> TRSGKVMRRLL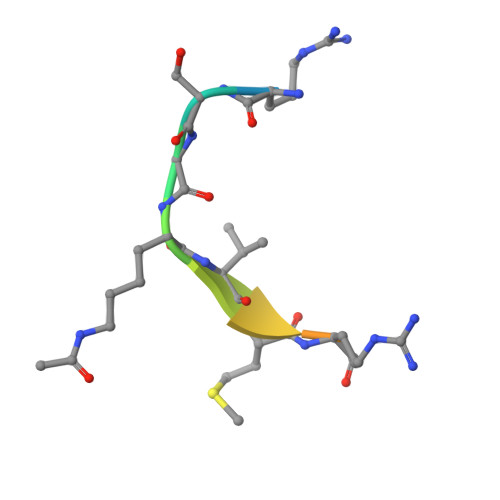R> 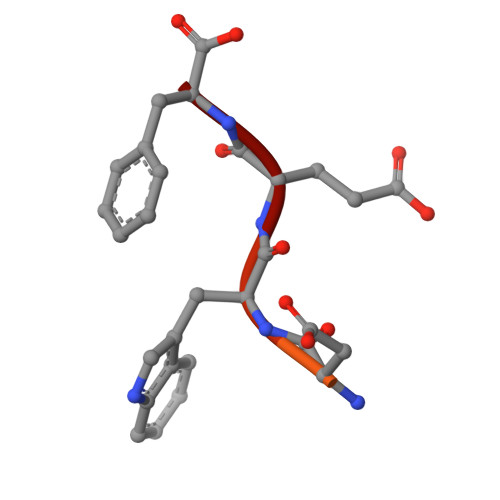NLEELEVDDWEF> GSFVEMVDNLRGKSGQGYYVEMTVGSPPQTLNILVDTGSSNFAVGAAPHPFLHRYYQRQLSSTYRDLRKGVYVPYTQGKWEGELGTDLVSIPHGPNVTVRANIAAITESDKFFINGSNWEGILGLAYAEIARPDDSLEPFFDSLVKQTHVPNLFSLQLCGAGFPLNQSEVLASVGGSMIIGGIDHSLYTGSLWYTPIRREWYYEVIIVRVEINGQDLKMDCKEYNYDKSIVDSGTTNLRLPKKVFEAAVKSIKAASSTE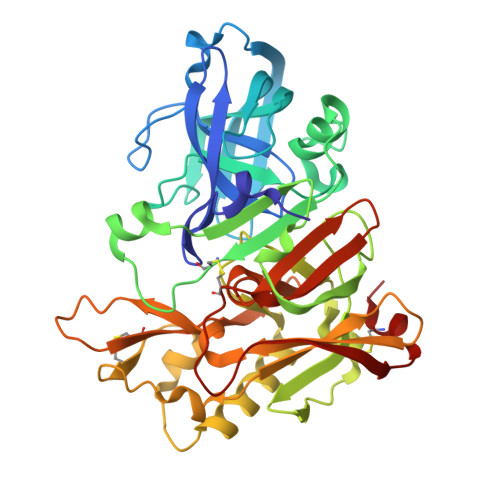KFPDGFWLGEQLVCWQAGTTPWNIFPVISLYLMGEVTNQSFRITILPQQYLRPVEDVATSQDDCYKFAISQSSTGTVMGAVIMEGFYVVFDRARKRIGFAVSACHVHDEFRTAAVEGPFVTLDMEDCGYN> MALDVKKYPFIKSLDDELKKYGGGITLTDLLLNSTTLIDQAKDRIQKTKSGDELPHYVSYNEPVLVFYTTLLSLAILNDVKLIRRYAYAEAKQFRSLLHTENEENLLEISKLLDLKINRCDPIKFYLEKKRRIIQKE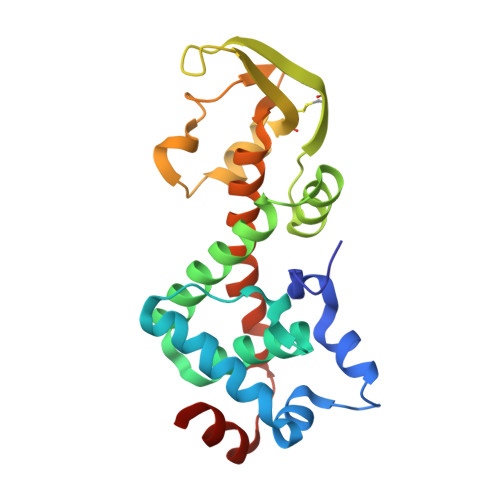FCVHFIDYLKYTKDLKEDWKLSGQILHKGYVYLDKNQLIGLIAESIKSKIVEMIRPLNLKEIPEKLKSLIERRGI>MDDEDNKCDCPPPGLPLWMGTFADLMSLLMCFFVLLLSFSEMDVLKFKQIAGSMKFAFGVQNQLEVKDIPKGTSIIAQEFRPGRPEPTPIDVIMQQTMDITQQTLEFHEGESDRAGGTKRDEGKLTGGQSPATSTQNNESAEADMQQQQSKEMSQEMETLMESIKKALEREIEQGAIEVENLGQQIVIRMREKGAFPEGSAFLQPKFRPLVRQIAELVKDVPGIVRVSGHTDNRPLDSELYRSNWDLSSQRAVSVAQEMEKVRGFSHQRLRVRGMADTEPLLPNDSDDNRALNRRVEISIMQGEPLYSEEVPVIQHHHHHH[2x];>[5x]MDLATLLGLIGGFAFVIMAMVLGGSIGMFVDVTSILIVVGGSIFVVLMKFTMGQFFGATKIAGKAFMFKADEPEDLIAKIVEMADAARKGGFLALEEMEINNTFMQKGIDLLVDGHDADVVRAALKKDIALTDERHTQGTGVFRAFGDVAPAMGMIGTLVGLVA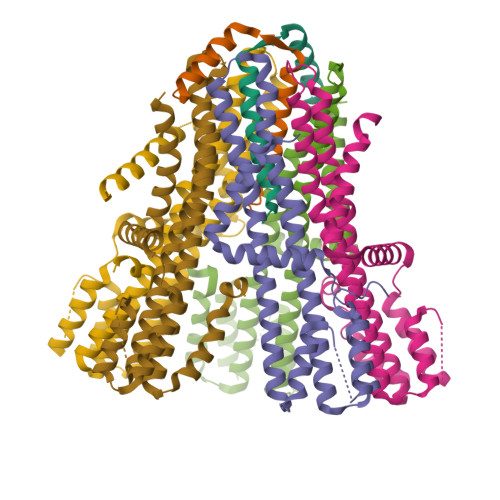MLSNMDDPKAIGPAMAVALLTTLYGAILSNMVFFPIADKLSLRRDQETLNRRLIMDGVLAIQDGQNPRVIDSYLKNYLNEGKRALEIDE>[3x]MFNLPPGNYKKPKLLYCSNGGHFLRILPDGTVDGTRDRSDQHIQLQLSAESVGEVYIKSTETGQYLAMDTDGLLYGSQTP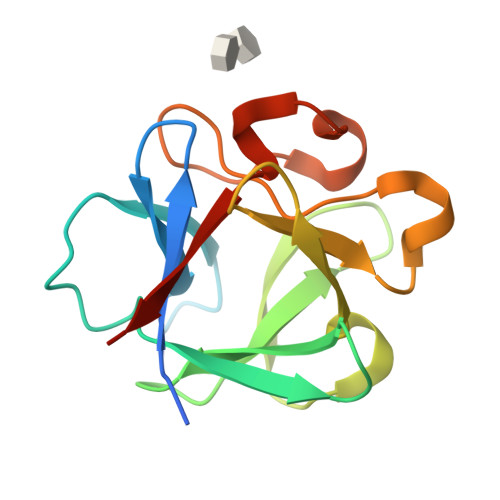NEECLFLERLEENHYNTYISKKHAEKNWFVGLKKNGSCKRGPRTHYGQKAILFLPLPVSSD>SKPQPIAAANWKSGSPDSLSELIDLFNSTSINHDVQCVVASTFVHLAMTKERLSHPKFVIAAQNAGNEDSLPSLKDFGVNWIVLGHSERRWYYGETNEIVADKVAAAVASGFMVIACIGETLQERESGRTAVVVLTQIAAIAKKLKKADWAKVVIAYEPVWAIGTGKVATPQQAQEAHALIRSWVSSKIGADVAGELRILYGGSVNG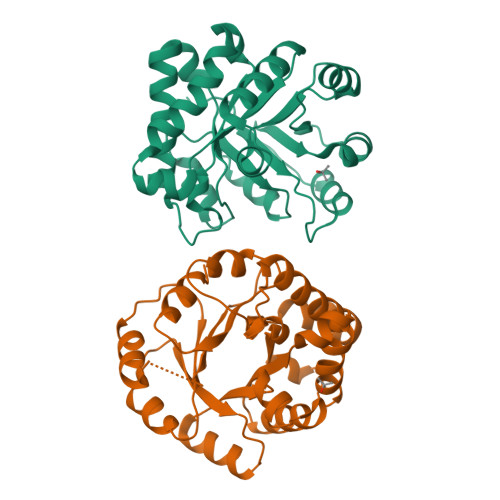KNARTLYQQRDVNGFLVGLKPEFVDIIKATQ[2x]>[2x]GSGAPPTDLQKMVMGNTKPVELNLDGKTVAICCATGVFGTAYLVPRHLFAE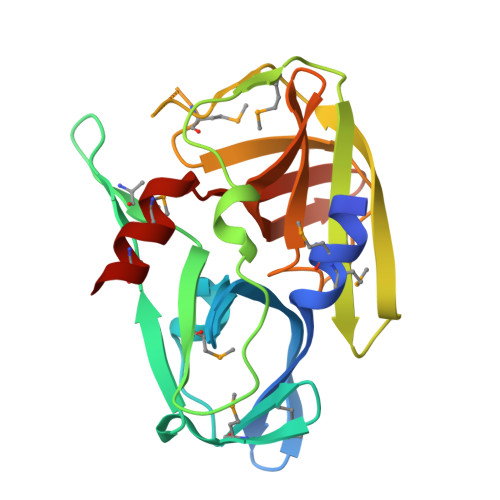KYDKIMLDGRAMTDSDYRVFEFEIKVKGQDMLSDAALMVLHRGNKVRDITKHFRDTARMKKGTPVVGVVNNADVGRLIFSGEALTYKDIVVSMDGDTMPGLFAYKAATRAGYAGGAVLAKDGADTFIVGTHSAGGNGVGYCSCVSRSMLQKMKAHVEH> MSFRKRGEILNDRGSGLRGPLLRGPPRTSSTPLRTGNRRAPGNVPLSDTTARLKKLNIADESKTKMGLDSSHVGVRPSPATSQPTTSTGSADLDSILGHMGLPLGNSVLVEEQSTTEFHSILGKLFAAQGIVHNRISDSSADKTRNGDTHVIVLSLNQMFAKELPGIYKGSRKQMKKNLISEEESKVTVQNLNETQRSTPSRYKDLKIAWKYKLADEKRLGSPDRDDIQQNSEYKDYNHQFDITTRLMPAPIASELTFIAPTQPVSTILSQIEQTIKRNDKKLIRIVIPSLLHPAMYPPKMFESSEIIGLMHGVRSLVKKYYERVVLFASISI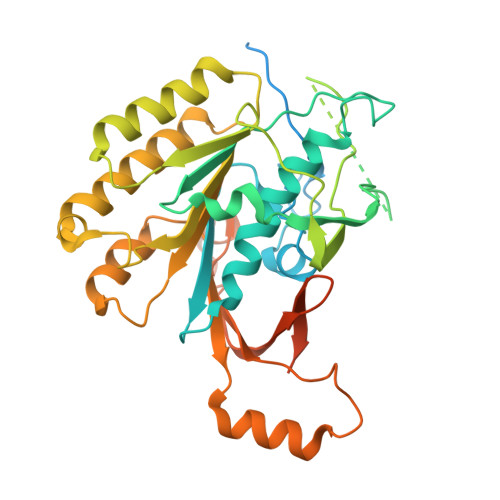DIITPPLLVLLRNMFDSVINLEPFNQEMTEFLERVYKSQPGKIQHGLVHILKLPVFTDRGEMRVLKSEWAFKNGRKKFEIEQWGIPVDDAEGSAASEQSHSHSHSDEISHNIPAKKTKISLDY Phosphoethanolamine (pEtN) cellulose is a naturally occurring modified cellulose produced by several Enterobacteriaceae. The minimal components of the E. coli cellulose synthase complex include the catalytically active BcsA enzyme, a hexameric semicircle of the periplasmic BcsB protein, and the outer membrane (OM)-integrated BcsC subunit containing periplasmic tetratricopeptide repeats (TPR). Additional subunits include BcsG, a membrane-anchored periplasmic pEtN transferase associated with BcsA, and BcsZ, a periplasmic cellulase of unknown biological function. Cellulose is a common bacterial biofilm component produced by a variety of prokaryotes, such as Escherichia coli (Ec), Salmonella enterica, and Gluconacetobacter/Komagataeibacter xylinus (Gx). These Gram-negative bacteria synthesize cellulose and secrete it across the cell envelope via the Bacterial cellulose synthase (Bcs) complex.

To gain experimental insights into the architecture of full-length BcsC and its interaction with cellulose by cryo-EM, we reconstituted the protein into a lipid nanodisc in the absence and the presence of cellotetraose. The obtained cryo-EM maps underscore the high flexibility of BcsC’s periplasmic domain. At lower contour levels and for the sample devoid of cellotetraose, the cryo-EM map confirms the solenoid architecture of TPR#9–19, while the N-terminal eight TPRs are insufficiently resolved or absent in the experimental map, Fig. 4a. Although the density cannot be identified unequivocally as a cello-oligosaccharide at the current resolution, its shape and interaction with BcsC are consistent with it representing a cellotetraose molecule, perhaps bound in different binding poses. Supporting this interpretation, no additional density at this site or elsewhere is observed in the absence of cellotetraose in a map of similar quality, Figs. 4b and S10. The cryo-EM structure of BcsC reveals that its periplasmic domain is flexibly attached to the β-barrel.

> MHHHHHHHHVEAAPTAQQQLLEQVRLGEATHREDLVQQSLYRLELIDPNNPDVVAARFRSLLRQGDIDGAQKQLDRLSQLAPSSNAYKSSRTTMLLSTPDGRQALQQARLQATTGHAEEAVASYNKLFNGAPPEGDIAVEYWSTVAKIPARRGEAINQLKRINADAPGNTGLQNNLALLLFSSDRRDEGFAVLEQMAKSNAGREGASKIWYGQIKDMPVSDASVSALKKYLSIFSDGDSVAAAQSQLAEQQKQLADPAFRARAQGLAAVDSGMAGKAIPELQQAVRANPKDSEALGALGQAYSQKGDRANAVANLEKALALDPHSSNNDKWNSLLKVNRYWLAIQQGDAALKANNPDRAERLFQQARNVDNTDSYAVLGLGDVAMARKDYPAAERYYQQTLRMDSGNTNAVRGLANIYRQQSPEKAEAFIASLSASQRRSIDDIERSLQNDRLAQQAEALENQGKWAQAAALQRQRLALDPGSVWITYRLSQDLWQAGQRSQADTLMRNLAQQKSNDPEQVYAYGLYLSGHDQDRAALAHINSLPRAQWNSNIQELVNRLQSDQVLETANRLRESGKEAEAEAMLRQQPPSTRIDLTLADWAQQRRDYTAARAAYQNVLTREPANADAILGLTEVDIAAGDKAAARSQLAKLPATDNASLNTQRRVALAQAQLGDTAAAQRTFNKLIPQAKSQPPSMESAMVLRDGAKFEAQAGDPTQALETYKDAMVASGVTTTRPQDNDTFTRLTRNDEKDDWLKRGVRSDAADLYRQQDLNVTLEHDYWGSSGTGGYSDLKAHTTMLQVDAPYSDGRMFFRSDFVNMNVGSFSTNADGKWDDNWGTCTLQDCSGNRSQSDSGASVAVGWRNDVWSWDIGTTPMGFNVVDVVGGISYSDDIGPLGYTVNAHRRPISSSLLAFGGQKDSPSNTGKKWGGVRADGVGLSLSYDKGEANGVWASLSGDQLTGKNVEDNWRVRWMTGYYYKVINQNNRRVTIGLNNMIWHYDKDLSGYSLGQGGYYSPQEYLSFAIPVMWRERTENWSWELGASGSWSHSRTKTMPRYPLMNLIPTDWQEEAARQSNDGGSSQGFGYTARALLERRVTSNWFVGTAIDIQQAKDYAPSHFLLYVRYSAAGWQGDMDLPPQPLIPYADW> MNELNNKMIEDVVLGEVELIEDLGQYFIDIEGDYEYNVEFATLSEVDYKVCALYEVATSKTYEVPYHDKLEKEDMKLFYDKWLEKDQQEETYIESVFFVNREDAESYIKDVLKGKESLTEVAAEIGYFE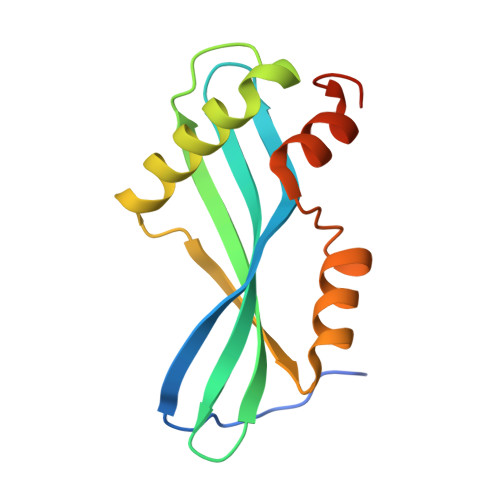LEHHHHHH> EEQW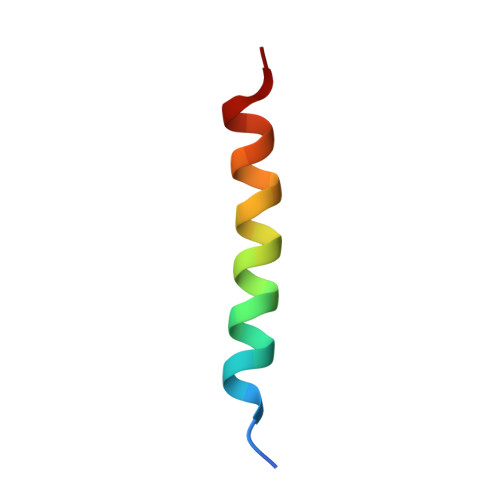AREIGAQLRRMADDLNAQYERR> SDTAPAGFQLERVVILSRHGVRAPTKMTQTMRDVTPHQWPEWPVKLGYITPRGEHLISLMGGFYRERFQQQGLLPKDNCPTPDAVYVWADVDQRTRKTGEAFLAGLAPQCDLAIHHQQNTQQADPLFHPVKAGICSMDKSQVHAAVEKQAGTPIETLNQRYQASLALMSSVLDFPKSPYCQQHNIGKLCDFSQAMPSRLAINDDGNKVALEGAVGLASTLAEIFLLEHAQGMPKVAWGNIHTEQQWNSLLKLHNAQFDLMSRTPYIAKHNGTPLLQTIAHALGSNITSRPLPDISPDNKILFIAGHDTNIANISGMLGMTWTLPGQPDNTPPGGALVFERWVDNAGKPYVSVNMVYQTLAQLHDQAPLTLQHPAGSVRLNIPGCSDQTPDGYCPLSTFSRLVSHSVEPACQLP

Phytases (myo-inositol hexakisphosphate phosphohydrolases) catalyse the hydrolysis of phytate into inorganic phosphate (Pi) and lower phosphorylated myo-inositols. Here we report the identification of two HAPPs from the enterobacteria Hafnia alvei (HaPhy) and Yersinia kristensenii (YkPhy), together with biochemical studies of their pH and temperature optima, as well as their phytate degradation pattern, which show that they are 6-phytases. The enzymes share a common catalytic site architecture located at the interface of the two domains involving the conserved N-terminal active site motif RHGXRXP and the C-terminal HD. The two-step reaction involves a nucleophilic attack on the phosphorous by the histidine from the RHGXRXP motif to form a covalent phosphohistidine intermediate while the aspartic acid of the HD motif serves as a proton donor to the oxygen atom of the scissile phosphomonoester bond.

The first attempt to co-crystallise HaPhy with the substrate analogue MIHS, at pH 8.4–9.1 led to the tar-HaPhy crystal. The structure was isomorphous to that of the apo-enzyme with the same disordered residues. The active site contained a tartrate molecule, a component of the crystallisation buffer and a well-known inhibitor of HAPs. The tartrate superimposes rather closely with the 6-sulphate moiety in the MIHS-HaPhy complex and the Pi in the Pi-YkPhy complex described below. There is a second tartrate, modelled with an occupancy of 0.25, close to a two-fold rotation axis, where it coordinates with His116 and Gln118 from two symmetry related HaPhy molecules. Perhaps it was not surprising that MIHS failed to bind at this high pH, since the optimal pH for HaPhy activity is ∼4.5 (see 4.1).> GKCGPPPPIDNGDITSFPLSVYAPASSVEYQCQ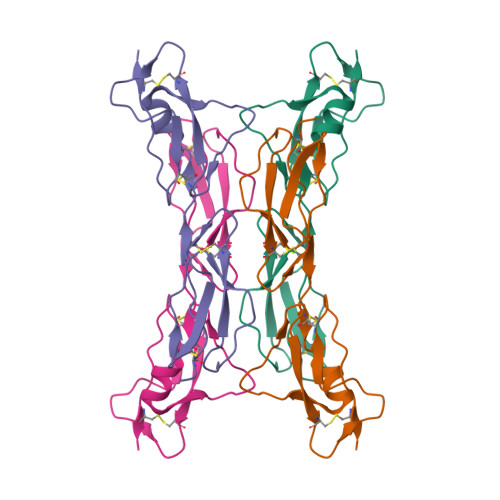NLYQLEGNKRITCRNGQWSEPPKCLHPCVISREIMENYNIALRWTAKQKLYSRTGESVEFVCKRGYRLSSRSHTLRTTCWDGKLEYPTCAKR> MRSHHHHHHGPGLVPRGSKTAAPVNALVSHLLVVEPEKLYAMPDPAGPDGHLPAVATLCDLFDREIVVTISWAKSIPGFSSLSLSDQMS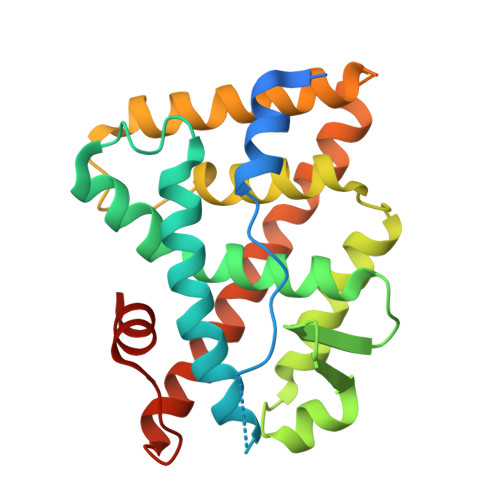VLQSVWMEVLVLGVAQRSLPLQDELAFAEDLVLDEEGARAAGLGELGAALLQLVRRLQALRLEREEYVLLKALALANSDSVHIEDAEAVEQLREALHEALLEYEAGRAGPGGGAERRRAGRLLLTLPLLRQTAGKVLAHFYGVKLEGKVPMHKLFLEMLEAMMD> HMTPPKAEKRPYPITTHGDTRVDDYYWLRDDERTDPQVLDYLQAENAFTDAALKPQQALRETLYEEMVARENLYFQSVPYVRHGYRYQTRFEPGNEYAIYVRQPQAESEHWDTLIDGNQRAEQREFYTLGGLEVSPDNQKLAVAEDFLSRRQYDIRFKNLSDDSWTDEVLENTSGSFEWANDSATVYYVRKHAKTLLPYQVYRHVVGTDPQLDELIYEEQDDTFYVGLEKTTSDRFILIHLSSTTTSEILLLDADRADSTPQMFVPRRKDHEYGIDHYHQHFYIRSNKDGKNFGLYQSEQADEAQWQTLIAPRIEVMLEGFSLFRDWLVVEERSEGLTQLRQIHWQSGEVKRIAFDDPTYTTWLAYNPEPETELLRYGYSSMTTPTTLYELNLDSDERVMLKQQEVKNFTPENYRSERVWVKARDGVEVPVSLVYRHDSFARGTNPLMVYGYGSYGSSMDPAFSASRLSLLDRGFVFVLAHIRGGGELGQLWYEDGKLFKKQNTFNDFIDVTEALIAQGYGDAKRVFAMGGSAGGLLMGAVINQAPELFNGIVAQVPFVDVVTTMLDESIPLTTGEYDEWGNPNQQAYYDYILQYSPYDQVKAQDYPHMLVTTGLHDSQVQYWEPAKWVAKLRELKTDDRQLLLYTDMDSGHGGKSGRFKAYEDIALEYAFILALAE

Oligopeptidase B (OpB) is a two-domain, trypsin-like serine peptidase belonging to the S9 prolyloligopeptidase (POP) family. Two domains are linked by a hinge region that participates in the transition of the enzyme between two major states—closed and open—in which domains and residues of the catalytic triad are located close to each other and separated, respectively. In this study, we described for the first time the structures of bacterial OpB from S. proteomaculans (PSP) obtained by X-ray for an enzyme with a modified hinge region (PSPmod) and two of its derivatives. The enzymes were crystallized in the presence of spermine and adopted uncommon intermediate states in the crystal lattices.

Finally, the tobacco etch virus (TEV) protease digestion site (ENLYFQ*S) was introduced by site-directed mutagenesis instead of amino acids 71-77 (IPQQEHS), forming the first hinge peptide. The hinge region modification included the substitution of the functionally important residue Glu75, which, according to our previous homology modeling and molecular dynamics studies, participated in the putative interdomain SB network stabilizing PSP in the closed conformation. PSPmod was crystallized in a conformation characterized by a disruption of the catalytic triad together with a domain arrangement intermediate between open and closed states found in crystals of ligand-free and inhibitor-bound POP, respectively. In the PSPmod structure, the distances between Cα-atoms in the pairs Ser532–His652 and His652–Asp617 are equal to 18.2 and 10.6 Å, respectively, which are longer than those in the closed states of TbOpB and ApPEP and comparable with those in the open state of TbOpB and intermediate states of PfPEP and GmPEP. In PSPmod, the His-loop location outside of the active center is stabilized by hydrophobic contacts of Met648 with Leu42, Glu43 and Asp46 residues of the α1-helix from the N-terminal loop. Gln619 was unable to form a SB with Arg151 and the latter interacted directly with catalytic Asp617, the interaction restricted His-loop movement and prevented rapprochement of His652 and Ser532 and consequent catalytic activation. In PSPmod, Sp702 is situated on the surface of the propeller domain near the η4-helix. Three Sp line the surface of the interdomain cavity of the catalytic (Sp703 and Sp705) and β-propeller (Sp701) domains, and Sp704 is located between the domains. Sp703 is remarkably close to catalytic Ser532: the distance 703C11-Ser532OG is 4.11 Å.> PDVVLVNGGEPPNPLIPTGTNDSNGGRIIDRLFAGLMSYDAVGKPSLEVAQSIESADNVNYRITVKPGWKFTDGSPVTAHSFVDAWNYGALSTNAQLQQHFFSPIEGFDDVAGAPGAASRTTMSGLRVVNDLEFTVRLKAPTIDFTLRLGHSSFYPLPDSAFRDMAAFGRNPIGNGPYKLADGPAGPAWEHNVRIDLVPNPDYHGNRKPRNKGLRFEFYANLDTAYADLLSGNLDVLDTIPPSALTVYQRDLGDHATSGPAAINQTLDTPLRLPHFGGEEGRLRRLALSAAINRPQICQQIFAGTRSPARDFTARSLPGFDPNLPGNEVLDYDPQRARRLWAQADAISPWSGRYAIAYNADAGHRDWVDAVANSIKNVLGIDAVAAPQPTFAGFRTQITNRAIDSAFRAGWRGDYPSMIEFLAPLFTAGAGSNDVGYINPEFDAALAAAEAAPTLTESHELVNDAQRILFHDMPVVPLWDYISVVGWSSQVSNVTVTWNGLPDYENIVKA;> SSVT

Herein, we show that heme and hemoglobin utilization converge at the cell surface of Mtb after heme is released from hemoglobin and demonstrate that the substrate-binding protein DppA is required for heme uptake across the inner membrane of Mtb. The components of the Mtb Dpp transporter include DppA (R3666c; substrate-binding protein), DppB/C (R3665c/Rv3664c, integral membrane permease proteins), and DppD (Rv3663c, ATPase). The substrate-binding protein DppA associated with the Dpp transporter binds heme with high affinity.

We obtained high-quality crystals of Mtb DppA that were used to determine a 3D-structure of the protein at 1.27 Å resolution. The atomic model of DppA, refined to an Rwork/free of 12.8/16.5%, sheds light on the molecular architecture of this periplasmic heme carrier with high accuracy. Mtb DppA has a globular shape that resembles a heart. Despite the compact appearance, the DppA tertiary structure is built by two globular and slightly offset halves that fold onto each other with perfect complementarity like the shells of a clam. The N-terminal half of the molecule (residues 1–249) connects to the C-terminal half (residues 267–541) by a flexible α-helical hinge (residues 250–266) that has higher than average B-factor in our structure (28.0 vs. 18.6 Å2). This hinge resembles a “clothespin spring” that keeps the two halves of DppA in a closed conformation poised to open up. Mtb DppA is similar to the homologous proteins found in Gram-negative bacteria, especially to the Salmonella typhimurium ortholog that superimposes to Mtb DppA with an RMSD ~1.45 Å. At the interface between the two DppA halves, completely buried inside the protein core, is a tetrapeptide whose amino acid sequence was modeled as Ser-Ser-Val-Thr. The electron density for this peptide is well-resolved, consistent with a tight binding. However, the physiological role of the tetrapeptide is unclear since DppAMtb was produced without the signal peptide in the cytoplasm of E. coli.> VTKPTIAAVGGYAMNNGTGTTLYTKAADTRRSTGSTTKIMTAKVVLAQSNLNLDAKVTIQKAYSDYVVANNASQAHLIVGD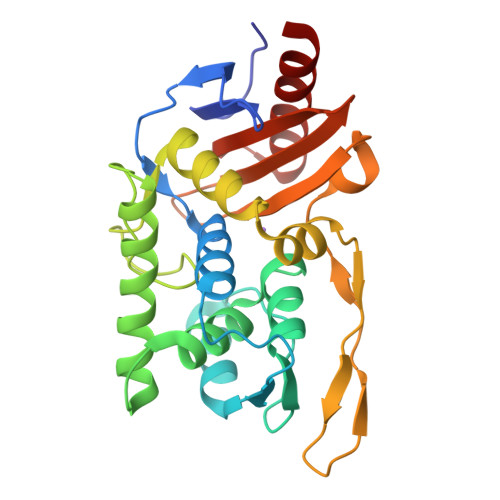KVTVRQLLYGLMLPSGADAAYALADKYGSGSTRAARVKSFIGKMNTAATNLGLHNTHFDSFDGIGNGANYSTPRDLTKIASSAMKNSTFRTVVKTKAYTAKTVTKTGSIRTMDTWKNTNGLLSSYSGAIGVKTGSGPEAKYCLVFAATRGGKTVIGTVLASTSIPARESDATKIMNYGFAL> GQDIQLIPPLINLLMSIEPDVIYAGHDNTKPDTSSSLLTSLNQLGERQLLSVVKWSKSLPGFRNLHIDDQITLIQYSWMSLMVFGLGWRSYKHVSGQMLYFAPDLILNEQRMKESSFYSLCLTMWQIPQEFVKLQVSQEEFLCMKVLLLLNTIPLEGLRSQTQFEEMRSSYIRELIKAIGLRQKGVVSSSQRFYQLTKLLDNLHDLVKQLHLYCLNTFIQSRALSVEFPEMMSEVI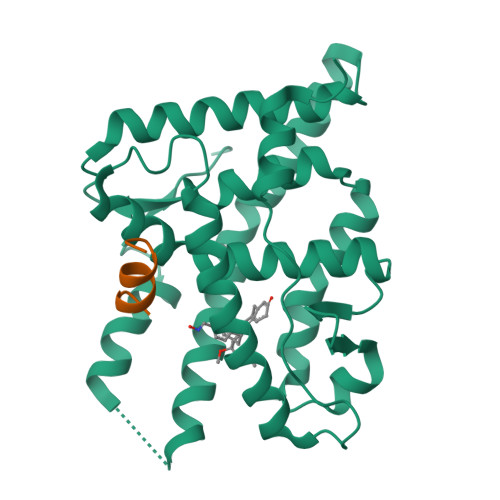AAQLPKILAGMVKPLLFHKK;> GHSFADPASNLGLEDIIRKALMGSF(2S,6S)-2,6-DIAMINO-2-METHYLHEPTANEDIOIC ACID | C8 H16 N2 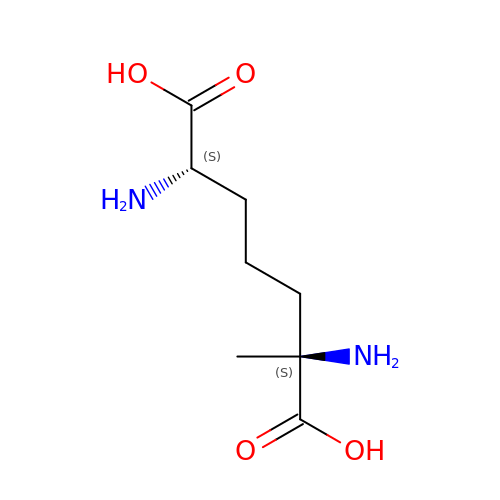O4 | TVZGBXIJPFGQBJ-XNCJUZBTSA-N> MEIPVIEPLFTKVTEDIPGAAGPVFDKNGDFYIVAPYVEVNGKPAGEILRIDLKTGKKTVICKPEVNGYGGIPAGCQCDRDANQLFVADARLGLLVVQTDGTFEEIAKKDSEGRRMQGCAYCAFDYEGNLWITAPAGEVAPADFTISLDEKFGSIYCFTTDGQMIQVDTAFQFPAGIAVRHMNDGRPYQLIVAEQRTKKLWSYDIKGPAKIENKKVWGHIPGTHEGGASGMDFDEDNNLLVANWGSSHIEVFGPDGGQPKMRIRCPFEKPSALHFKPQTKTIFVTEHENNAVWKFEWQRNGKKQYC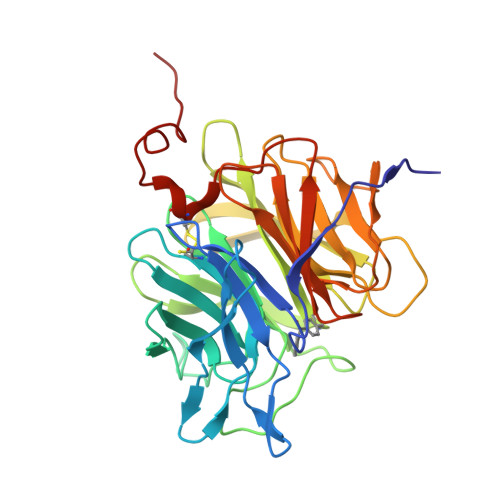ETLKFGIFGSLEHHHHHH2'-(2-fluorophenyl)-1-methyl-6',8',9',11'-tetrahydrospiro[azetidine-3,10'-pyrido[3',4':4,5]pyrrolo[2,3-f]isoquinolin]-7'(5'H)-one 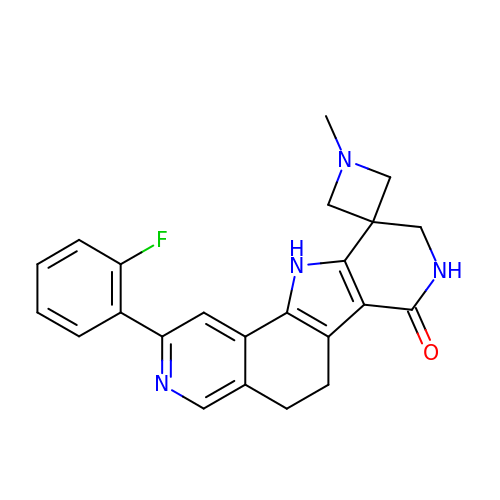| C23 H21 F N4 O | XZZOJFOFCDHYRX-UHFFFAOYSA-N> MGKYNLILSEYLSFIYNSQSAVQIPIYYSSNSELENRCIEFHSKCLENSKNGLSLKKLFVEYSDVIENATLLSILSYSYDKYNAVERKLVKYAKGKPLEADLTVNELDYENNKITSELFPTAEEYTDLLMDPAILTSLSSNLNAVMFWLEKHENDVAEKLKIYKRRLDLFTIVASTVNKYGVPRHNAKYRYEYEVMKDKPYYLVTWANSSIEMLMSVFSHEDYLIARELIVLSYSNRSTLAKLVSSPMSILVALVDINGTFITNEELELEFSNKYVRAIVPDQTFDELKQMLDNMRKAGLTDIPKMIQDWLVDCSIEKFPLMAKIYSWSFHVGFRKQKMLDAALDQLKTEYTEDVDDEMYREYTMLIRDEVVKMLEEPVKHDDHLLQDSELAGLLSMSSASNGESRQLKFGRKTIFSTKKNMHVMDDMANGRYTPGIIPPVNVDKPIPLGRRDVPGRRTRIIFILPYEYFIAQHAVVEKMLIYAKHTREYAEFYSQSNQLLSYGDVTRFLSNNSMVLYTDVSQWDSSQHNTQPFRKGIIMGLDMLANMTNDARVIQTLNLYKQTQINLMDSYVQIPDGNVIKKIQYGAVASGEKQTKAANSIANLALIKTVLSRISNKYSFATKIIRVDGDDNYAVLQFNTEVTKQMVQDVSNDVRETYARMNTKVKALVSTVGIEIAKRYIAGGKIFFRAGINLLNNEKKGQSTQWDQAAVLYSNYIVNRLRGFETDREFILTKIMQMTSVAITGSLRLFPSERVLTTNSTFKVFDSEDFIIEYGTTDDEVYIQRAFMSLSS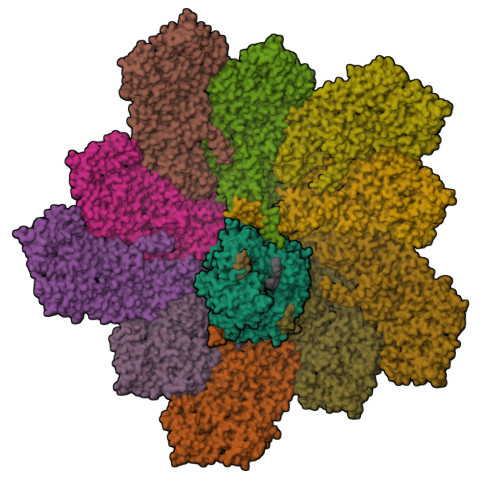QKSGIADEIAASSTFKNYVSRLSEQLLFSKNNIVSRGIALTEKAKLNSYAPISLEKRRAQISALLTMLQKPVTFKSSKITINDILRDIKPFFTVNEAHLPIQYQKFMPTLPDNVQYIIQCIGSRTYQIEDDGSKSAISRLISKYSVYKPSIEELYKVISLHENEIQLYLISLGIPKIDADTYVGSKIYSQDKYRILESYVYNLLSINYGCYQLFDFNSPDLEKLIRIPFKGKIPAVTFILHLYAKLEVINHAIKNGSWISLFCNYPKSEMIKLWKKMWNITSLRSPYTNANFFQD;>[10x]MAYRKRGARRETNLKQDDRMQEKEENKNVNTNSENKNATKPQLSEKVLSQKEEVITDNQEEIKIADEVKKSNKEESKQLLEVLKTKEEHQKEVQYEILQKTIPTFEPKESILKKLEDIKPEQVKKQTKLFRIFEPRQLPVYRANGEKELRNRWYWKLKRDTLPDGDYDVREYFLNLYDQVLTEMPDYLLLKDMAVENKNSRDAGKVVDSETAAICDAIFQDEETEGVVRRFIAEMRQRVQADRNVVNYPSILHPIDHAFNEYFLQHQLVEPLNNDIIFNYIPERIRNDVNYILNMDRNLPSTARYIRPNLLQDRLNLHDNFESLWDTITTSNYILARSVVPDLKELVSTEAQIQKMSQDLQLEALTIQSETQFLTGINSQAANDCFKTLIAAMLSQRTMSLDFVTTNYMSLISGMWLLTVVPNDMFIRESLVACQLAIINTIIYPAFGMQRMHYRNGDPQTPFQIAEQQIQNFQVANWLHFVNNNQFRQVVIDGVLNQVLNDNIRNGHVVNQLMEALMQLSRQQFPTMPVDYKRSIQRGILLLSNRLGQLVDLTRLLAYNYETLMACITMNMQHVQTLTTEKLQLTSVTSLCMLIGNATVIPSPQTLFHYYNVNVNFHSNYNERINDAVAIITAANRLNLYQKKMKSIVEDFLKRLQIFDISRVPDDQMYRLRDRLRLLPVEIRRLDIFNLILMNMEQIERASDKIAQGVIIAYRDMQLERDEMYGYVNIARNLDGFQQINLEELMRTGDYAQITNMLLNNQPVALVGALPFITDSSVISLVAKLDATVFAQIVKLRKVDTLKPILYKINSDSNDFYLVANYDWVPTSTTKVYKQIPQQFDFRASMHMLTSNLTFTVYSDLLAFVSADTVEPINAVAFDNMRIMNEL>ISEFDSEGSNMSTTAHTEPSWADLPFLDFTDPNFSWDSPEVAEAREKSWIARTPLALLVLRYAEADQLARDKRLISGFRGLVDMVGTPEGPVRDFMVDFLQSLDGADHRRLRGLATHPFTPRRITAVQPFVRSTVEQLIDKLPQGDFDFVQHFPHPLPALVMCQLLGFPLEDYDTVGR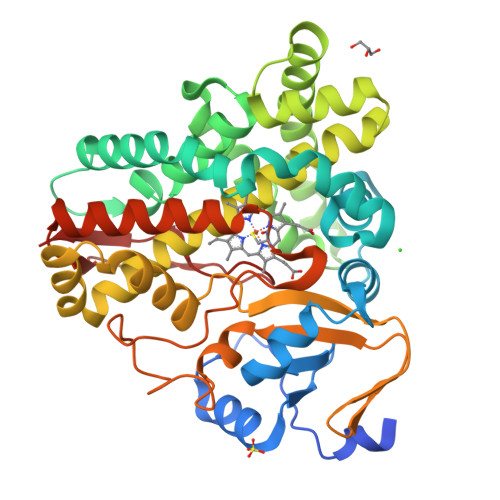LSIETNLGLALSNDQDILVKVEQGLGRMFDYLVAAIEKRKVEPGDDLTSDIVRAFHDGVLDDYELRTLVATVLVAGYETTNHQLALAMYDFAQHPDQWMKIKENPELAPQAVEEVLRWSPTLPVTATRVAAEDFEVNGVRIPTGTPVFMCAHVAHRDPRVFADADRFDITVKREAPSIAFGGGPHFCLGTALARLELTEAVAALATRLDPPQIAGEITWRHELGVAGPDALPLRFGAA[2x]3-CHLORO-BENZAMIDE | C7 H6 Cl N O 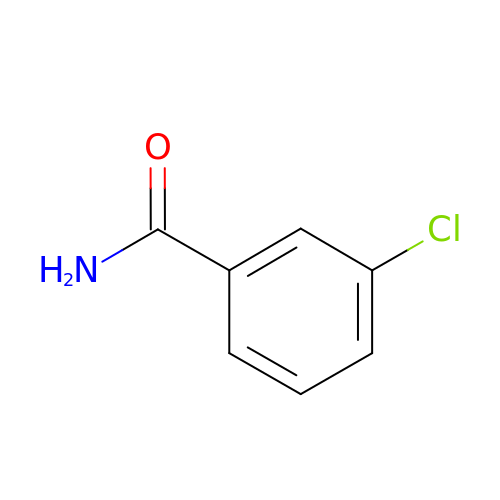| MJTGQALMWUUPQM-UHFFFAOYSA-N ADP-ribosylation is a reversible post-translational modification involved in various cellular activities. Removal of ADP-ribosylation requires (ADP-ribosyl)hydrolases, with macrodomain enzymes being a major family in this category. Further analyses reveal DUF4804 as a class of MavL-like macrodomain enzymes whose representative members show unique selectivity for mono-ADP-ribosylated arginine residue in synthetic substrates. Crystal structures of several proteins in this class provide insights into arginine specificity and a shared mode of ADP-ribose interaction distinct from previously characterized macrodomains.

Thus, it appears that the arginine insertion contributes to packing interactions outcompeting ADPR binding. Mutation of R370 to alanine, while retaining normal (ADP-ribosyl)hydrolase activity, led to successful capture of ADPR-bound MavL, with well-defined electron density guiding unambiguous placement of the ligand. H142 and Y265 interact with the adenosine via π-π stacking, yet a commonly present aspartate in other macrodomains stabilizing the N6 atom of adenosine is absent in MavL. Furthermore, the proximal ribose is held by interactions with the backbone of G221 and P264 and the side chains of T224 and K236. The di-phosphate mainly interacts with the backbone atoms of the loop containing residues from G223 to F227 (referred to here as the di-phosphate binding loop, loop 1): specifically, the α-phosphate with C226 and D332 and the β-phosphate with G223, G225, and F227. Another loop from D315 to D323 (referred to here as the catalytic loop, loop 2) is responsible for the distal ribose binding in MavL, with D315, N322, and D323 directly forming hydrogen bonds with hydroxyl groups on the C3”, C2” and C3”, and C1” atoms, respectively. In addition, D333 forms hydrogen bonds to the hydroxyl group on the C2” atom. Mutations of D315, D323, D333, or F227, to alanine resulted in a significant loss of activities of MavL, whereas N322A and T331A mutants only exhibited activity loss with low enzymatic concentrations. From the same structure, we observed five ordered waters around the distal ribose, three of them (w1, w2, and w3) above and two (w4 and w5) below the ribose ring. On the other hand, the substrate-associated w4 is bound to the phosphate groups of the ADPR and further stabilized by the backbone of A313 and D333, and the side chain of T331. This water is the closest to C1” atom (with a distance of 3.3 Å); accordingly, we propose it to be the catalytic water and its possible activation by the α-phosphate of ADPR for nucleophilic attack at the C1” center following an SN2 mechanism.

> GPLGSAYQLLLSKETLNKILQYKQNLEKGLATPGKFFLEELSKQEKSISEMDITTFTQLLIQSKKPQVFAESQVYHDGTDWTLEEESILGDVSVNMPVTMYNDGGHGSSFKNHPKPISGYLAYVPGALLASGSGPTSDMKEVLDNGKLNQDKLNALYERRLLPQLIHFNELARQNEKQAAITIPGIGTGCFSGAYYDVIKPYVRNALIHILEKHKDSLPYIDIIHYDPYMGDEPAEKKIGHMSFRVSPSGVVRGTTGQLDYPLGSNPDTHILVSIVAWDHFSWPGNDYWGGARQTDDGVKAASTDTMGQVTGATGVYDKKWGRYMPPESFTKDAKGMSDWGDYVRENGIVFNGPVLALDKSGKLDTLENVASRSSKAKVETTTTISDLVRSMFSLFSHS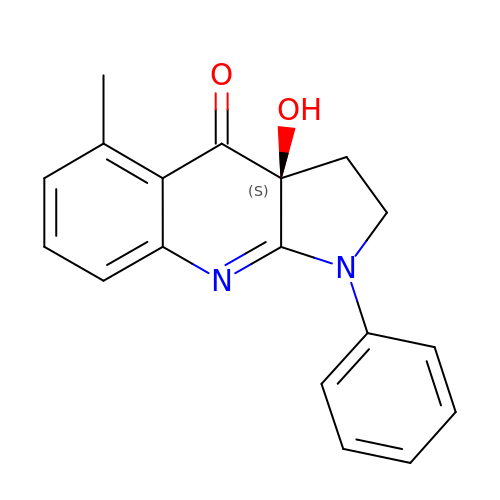(3aS)-3a-hydroxy-5-methyl-1-phenyl-1,2,3,3a-tetrahydro-4H-pyrrolo[2,3-b]quinolin-4-one | C18 H16 N2 O2 | NJBBBRZNBVLTRZ-GOSISDBHSA-N>[2x]MARKYFVAANWKCNGTLESIKSLTNSFNNLDFDPSKLDVVVFPVSVHYDHTRKLLQSKFSTGIQNVSKFGNGSYTGEVSAEIAKDLNIEYVIIGH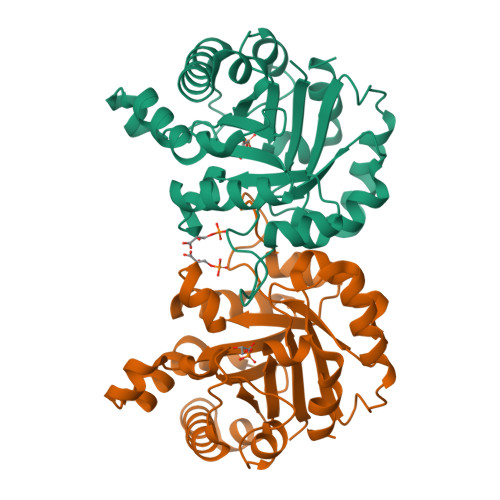FERRKYFHETDEDVREKLQASLKNNLKAVVCFGESLEQREQNKTIEVITKQVKAFVDLIDNFDNVILVYEPLWAIGTGKTATPEQAQLVHKEIRKIVKDTCGEKQANQIRILYGGSVNTENCSSLIQQEDIDGFLVGNASLKESFVDIIKSAM> GSHMAASQTSQTVASHVPFADLCSTLERIQKSKGRAEKIRHFREFLDSWRKFHDALHKNHKDVTDSFYPAMRLILPQLERERMAYGIKETMLAKLYIELLNLPRDG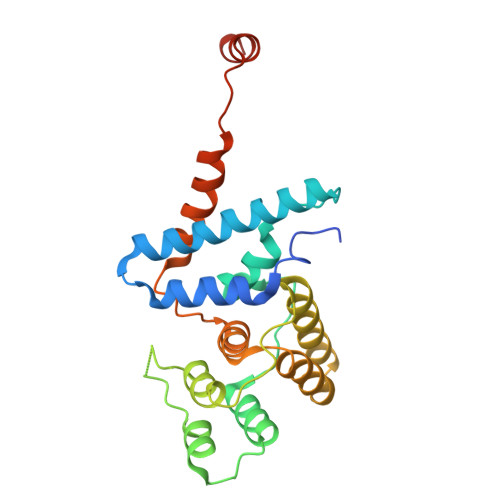KDALKLLNYRTPTGTHGDAGDFAMIAYFVLKPRCLQKGSLTIQQVNDLLDSIASNNSAKRKDLIKKSLLQLITQSSALEQKWLIRMIIKDLKLGVSQQTIFSVFHNDAAELHNVTTDLEKVCRQLHDPSVGLSDISI> MPINIRRATINDIICMQNANLHNLPENYMMKYYMYHILSWPEASFVATTTT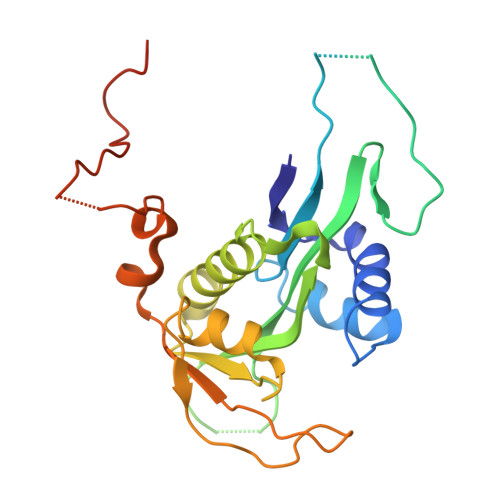LDCEDSDEQDENDKLELTLDGTNDGRTIKLDPTYLAPGEKLVGYVLVKMNDDPDQQNEPPNGHITSLSVMRTYRRMGIAENLMRQALFALREVHQAEYVSLHVRQSNRAALHLYRDTLAFEVLSIEKSYYQDGEDAYAMKKVLKLEELQISNFTHRRLKENEEKLEDDLESDLLEDIIKQGVNDIIV> MATHDIAAQHLADGIAASGPAPDLAAAAAFLEMGDRLGVVAHLDPDRTLETAEVAAALDLPEPALVRYLDAVESAGLVIREGEGRYRACPDFDTIRHQAGYISWTMNANRPFIENARDFFTDWDKAARTHVRDYREVAVSSQWMGSHAFYPTALATIIDAAPRKVVDLGAGTCRLLIEVLGAVPGSTGVGLDFAADACRAAEQAVAQAGMTDRLTVVERTIQSVATDPGVLEGADVIHAGFVFHDMLPEEEDVCDQVLANCRESLAPGGFLAITDAVPYLRNDRERRFSAAVSYYHGEFMRRRLQSEEEWVERLRGAGFSDVRALTLAFPTGRLFLAHR

SgvM is found in the biosynthetic gene cluster of the antibiotic viridogrisein and catalyzes methyl transfer to the C3 (i.e., β) position of α-ketoleucine (4-methyl-2-oxovalerate). The overall structure consists of a two-domain fold that assembles into homodimer in both the solution and the crystal. The N-terminal domain (I6 through H147) consists of helices that mediate dimerization, while the C-terminal domain (F149 through H338) consists of a Rossman fold. A single metal ion is located at the base of the C-terminal domain and is ligated by H244 and H296.

Hence, we first determined the 2.13 Å resolution structure of wt SgvM in complex with MTA and α-ketoleucine. Density corresponding to the α-ketoleucine substrate can be observed directly bound to the metal. However, SAM could not be observed in the structure but rather density for MTA, likely derived from SAM hydrolysis, is seen in the near vicinity of the metal. The distance from the MTA sulfur atom to C3 position of α-ketoleucine is ca. 7 Å, suggesting that this represents a nonproductive complex. This non-productive complex resembles that observed in the previously reported structure of SgvM. Anomalous difference Fourier maps calculated from data collected at the zinc absorption edge, and the tetrahedral coordination are consistent with a bound zinc ion. The zinc is likely integral to the enzyme as no exogenous metals were added during purification or crystallization. Presumably, the metal ion acts as a Lewis acid to trigger the soft enolization of the ketoacid substrate and facilitates electrophilic methylation.>[4x]MNHLRAEGPASVLAIGTANPENILLQDEFPDYYFRVTKSEHMTQLKEKFRKICDKSMIRKRNCFLNEEHLKQNPRLVEHEMQTLDARQDMLVVEV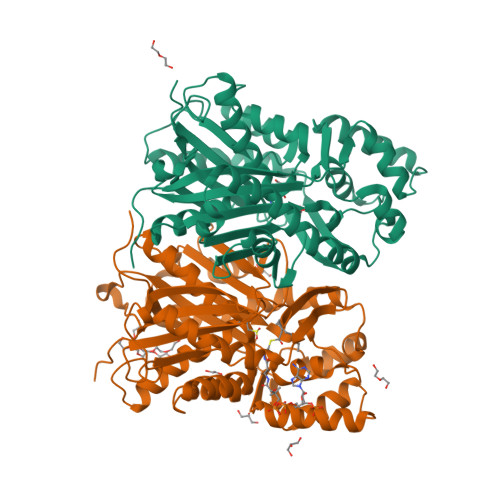PKLGKDACAKAIKEWGQPKSKITHLIFTSASTTDMPGADYHCAKLLGLSPSVKRVMMYQLGCYGGGTVLRIAKDIAENNKGARVLAVCCDIMACGFRGPSESDLELLVGQAIFGDGAAAVIVGAEPDESVGERPIFELVSTGQTILPNSEGTIGGHIREAGLIFDLHKDVPMLISNNIEKCLIEAFTPIGISDWNSIFWITHPGGKAILDKVEEKLHLKSDKFVDSRHVLSEHGNMSSSTVLFVMDELRKRSLEEGKSTTGDGFEWGVLFGFGPGLTVERVVVRSVPIKY>MAHHHHHHMSERLKDRVALVTGAASGIGAATARLMAQEGAFVVLADVDEHAGQALARELRDATFAYTDVSVEAQVAAAVDEALRLHGRLDCMVNNAGFVGAYGSILETSAAAWHATLGVLLDGVFYGIKHAARAMVKQGSGCILSVASTAGVMGGLGPHAYTSAKHAVIGLTRSAASELAP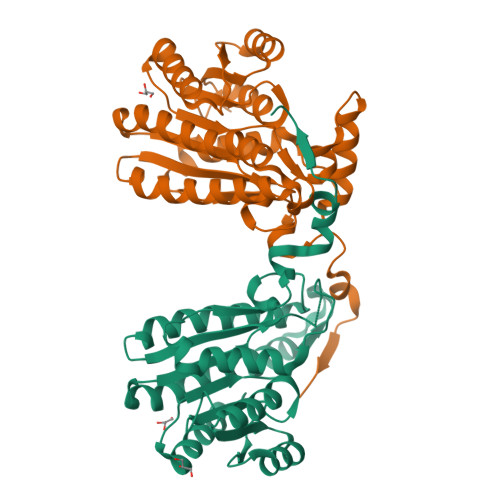RGVRVNAVAPGTTVTEMMVQGRGSRQAAIDAATRASPLGTPLMPQEIAAALVYLASDDARHVNAHTLVVDSGVTVAGASGGAVFHNRPAGFMGRMPGGANADAR[4x]>MSLQNMETRYTHSPADIRHYSTEQLRDEFLVEKVFIPGAISLTYTHNDRMIFGGVTPTTEELEIILDKELGVDYFLERRELGVINIGGPGFIEIDGAKETMKKQDGYYIGKETKHVRFSSENPDNPAKFYISCVPAHHKYPNVKISIDEITPMETGDPLTLNQRKIYQYIHPNVCES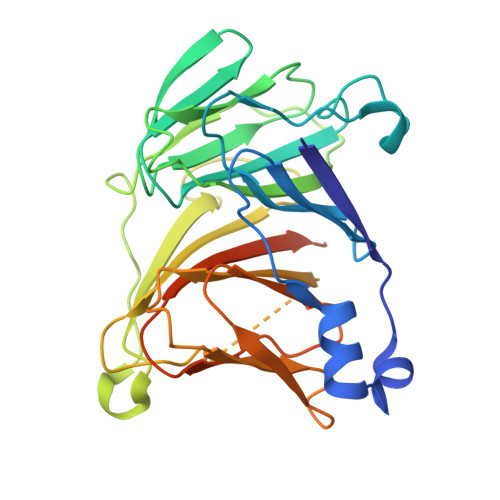CQLQMGYTILEPGSAWNTMPCHTHERRMEAYVYFDMEEDTRIFHMMGKPDETKHLVMSNEQAAISPSWSIHSGVGTSNYSFIWAMCGENITYTDMDMVAMDQLKEGHHHHHH[6x]3-{5-[(2E,4aR,7aR)-2-imino-6-(3-methoxypyridin-2-yl)-3-methyl-4-oxooctahydro-7aH-pyrrolo[3,4-d]pyrimidin-7a-yl]thiophen-3-yl}benzonitrile 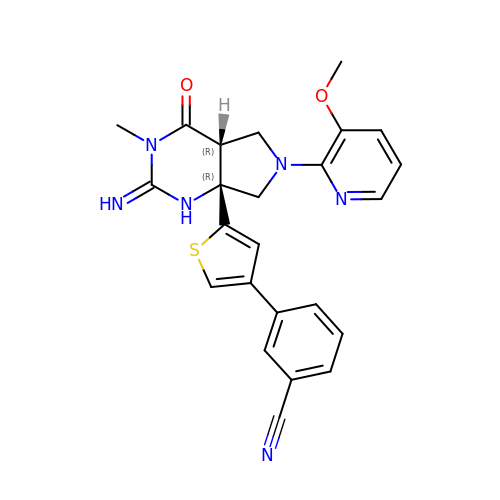| C24 H22 N6 O2 S | OVZBZLASXPSCEA-UUOWRZLLSA-N>PVTLTLYNGQHAATGIAIAKAFQDKTGIQVKIRKGGDGQLASQITEEGARSPADVLY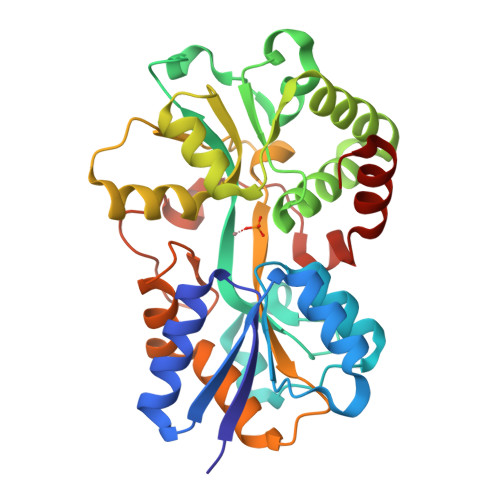TEESPPLIRLASAGLLAKLEPETLALVEPEHAGGNGDWIGITARTRVLAYNPKKIDEKDLPKSLMDLSDPSWSGRFGFVPTSGAFLEQVAAVIKLKGQEEAEDWLTGLKAFGSIYTNNVTAMKAVENGEVDMALINNYYWYTLKKEKGELNSRLHYFGNQDPGALVTVSGAAVLKSSKHPREAQQFVAFMLSEEGQKAILSQSAEYPMRKGMQADPALKPFAELDPPKLTPADLGEASEALSLERDVGLN[2x]> MNDHIHRVPALTEEEIDSVAIKTFERYALPSSSSVKRKGKGVTILWFRNDLRVLDNDALYKAWSSSDTILPVYCLD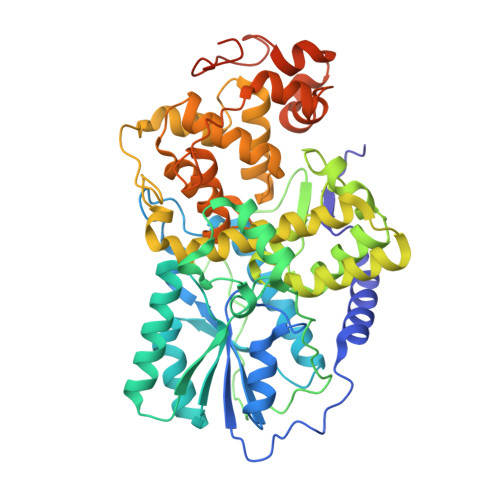PRLFHTTHFFNFPKTGALRGGFLMECLVDLRKNLMKRGLNLLIRSGKPEEILPSLAKDFGARTVFAHKETCSEEVDVERLVNQGLKRVGNSTKLELIWGSTMYHKDDLPFDVFDLPDVYTQFRKSVEAKCSIRSSTRIPLSLGPTPSVDDWGDVPTLEKLGVEPQEVTRGMRFVGGESAGVGRVFEYFWKKDLLKVYKETRNGMLGPDYSTKFSPWLAFGCISPRFIYEEVQRYEKERVANNSTYWVLFELIWRDYFRFLSIKCGNSLFHLGGPRNVQGKWSQDQKLFESWRDAKTGYPLIDANMKELSTTGFMSNRGRQIVCSFLVRDMGLDWRMGAEWFETCLLDYDPCSNYGNWTYGAGVGNDPREDRYFSIPKQAQNYDPEGEYVAFWLQQLRRLPKEKRHWPGRLMYMDTVVPLKHGNGPMAGGSKSGGGFRGSHSGRRSRHNGP>MFNMNVDESASGALGSSAIPVHPTPASVRLFEILQGKYAYVQGQTIYANLRNPGVFSRQVFTHLFKRAISHCTYDDVLHDWNKFEACIQKRWPSDDSCASRFRESTFESWSTTMKLTVRDLLTTNIYRVLHSRSVLSYERYVDWICATGMVPAVKKPITQELHSKIKSLRDRCVCRELGHERTIRSIGTELYEATKEIIESLNSTFIPQFTEVTIEYLPRSDEYVAYYCGRRIRLHVLFPPAIFAGTVTFDSPVQRLYQNIFMCYRTLEHAKICQLLNTAPLKAIVGHGGRDMYKDILAHLEQNSQRKDPKKELLNLLVKLSENKTISGVTDVVEEFITDASNNLVDRNRLFGQPGETAAQGLKKKVSNTVVKCLTDQINEQFDQINGLEKERELYLKKIRSMESQLQASLGPGGNNPAASAPAAVAAEAASVDILTGSTASAIEKLFNSPSASLGARVSGHNESILNSFVSQYIPPSREMTKDLTELWESELFNTFKLTPVVDNQGQRLYVRYSSDTISILLGPFTYLVAELSPVELVTDVYATLGIVEIIDELYRSSRLAIYIEDLGRKYCPASATGGDHGIRQAPSARGDTEPDHAKSKPARDPPPGAGS[12x]

Epstein-Bar virus (EBV), a member of the subfamily gammaherpesviruses that also includes the Kaposi Sarcoma-associated herpesvirus (KSHV),2,3 is the first identified oncovirus. Similar to other members of the family herpesviridae, EBV has a characteristic three-layer configuration: the outer lipid bilayer envelope containing viral glycoproteins responsible for host recognizing and membrane fusion, the inner pseudo-icosahedral nucleocapsid enclosing a 172-kb double-strand DNA (dsDNA) genome and the middle pleomorphic tegument compartment fulfilled with 20–40 different viral proteins. All herpesvirus capsid shell consists of 4 abundant proteins: the major capsid proteins (MCP) constituting the basic capsid skeleton through forming 150 hexons and 11 pentons, the small capsid proteins (SCP) binding to the tops of hexon MCPs or both hexon and penton MCPs, and the Tri1 and Tri2 forming the heterotrimeric triplexes to plug the large holes on the capsid floor. Once the viral dsDNA genome enters the procapsid shell through the portal that is located at a unique 5-fold vertex of the icosahedral capsid, the viral nucleocapsid is joined by the capsid-associated tegument complexes (CATCs).

Based on the density map of the C12 portal reconstruction, we built an atomic model of the portal protein BBRF1. The portal channel has two narrow regions that interact directly with the terminal DNA. The first one, located at the interface between the stem and crown domains, is the channel valve formed by 12 copies of β-hairpins protruding toward the channel axis. The channel valve is the most constricted region of the portal channel, with a diameter of ~25 Å. Similar to the counterparts in tailed bacteriophages, the channel valve of the EBV portal should play key roles in DNA retention and ejection. The second narrow region is a tunnel-like structure composed of 12 sets of three-stranded β-sheets radially arranged around the channel axis, with a diameter of 31 Å. Each β-sheet is formed through β-augmentation between a β-strand from the clip domain of one BBRF1 monomer and a two-parallel-stranded β-sheet from the clip base of its counterclockwise neighbor (viewing toward the capsid interior). The portal-DNA interactions are contributed mainly by four basic residues (H79, K90, R155 and R176) of BBRF1. Compared to the in vitro-assembled EBV portal, our in situ portal exhibited a more compact conformation with gradually decreased interior diameters from the clip region (31 Å vs 31 Å) downward through the channel valve (25 Å vs 32 Å) to the crown region (58 Å vs 75 Å). Consequently, the terminal DNA of the packaged genome in the mature EBV capsid is firmly held by the significantly narrowed portal channel valve, which would further alleviate the pressure placed on the portal cap.>GPEDDHHMEFCRVCKDGGELLCCDTCPSSYHIHCLNPPLPEIPNGEWLCPRCTCPALKGKVQKILIWKWGQPPSPTPVPRPPDADPNTPSPKPLEGRPERQFFVKWQGMSYWHCSWVSELQLELHCQVMFRNYQRKNDMDEPPSGDFGGDEEKSRKRKNKDPKFAEMEERFYRYGIKPEWMMIHRILNHSVDKKGHVHYLIKWRDLPYDQASWESEDVEIQDYDLFKQS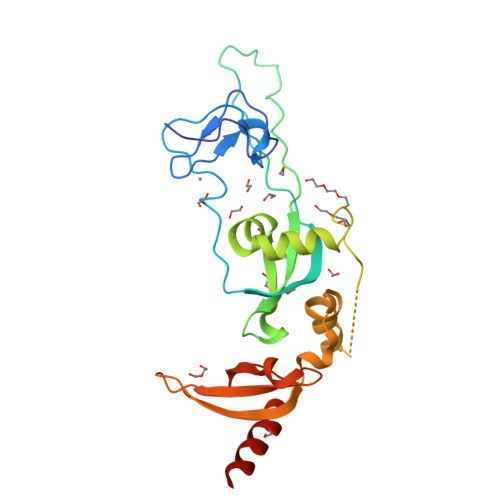YWNHRELMR[4x]McrBC is a two-component MDRS that in Escherichia coli (Ec) restricts phage DNA and foreign DNA containing methylated cytosines. EcMcrB consists of an N-terminal DNA-binding domain that targets fully or hemi-methylated RMC sites (where R is a purine base and MC is a 4-methyl-, 5-methyl-, or 5-hydroxymethyl-cytosine), and a C-terminal AAA+ (extended ATPases Associated with various cellular Activities) domain that hydrolyzes GTP and oligomerizes into hexamers. Biochemical data suggest that stimulated GTP hydrolysis powers DNA translocation, allowing EcMcrBC complexes bound to distant RMC sites to interact and induce cleavage on both strands. Here, we present cryo-EM structures of an McrB hexamer and McrBC complexes from the evolutionarily distant archaeal species Thermococcus gammatolerans (Tg) and the well-characterized E. coli system.

To overcome this limitation, we produced complexes containing full-length TgMcrC bound to the AAA+ domain of TgMcrB (TgMcrBAAAC) in the presence of GTPγS. This assembly was structurally more homogeneous and allowed us to calculate maps of the “half”-complex at 3.7-Å resolution, as well as a C2-symmetrized map of the entire TgMcrBAAAC tetradecameric complex at 4.2-Å resolution. A TgMcrC dimer bridges two TgMcrBAAA hexamers in this structure, with the scaffold and nuclease domains forming the dimer interface. The nuclease domains associate through their α12 helices and a loop between the β10 and β11 strands (“L”), whereas the neighboring scaffold domains interact with each other through their β4 strands that form main-chain hydrogen bonds with each other. Structural superposition confirms TgMcrC’s C terminus shares the same fold and identifies Asp340TgMcrC, Asp354TgMcrC, and Lys356TgMcrC as putative catalytic side chains based on their spatial alignment with the EndoMS metal-binding residues. The nuclease domains align in an orientation that resembles the dimer configuration captured in our cryo-EM structures; however, we observe numerous steric clashes in both models. TgMcrC’s scaffold domain and the α12 nuclease helices collide with the DNA substrate. We therefore speculate that our dimeric McrBC structures depict a conformation that is incompatible with DNA cleavage, and that a major conformational change would be required for nuclease activity to proceed unencumbered. Modeling these interactions in the context of the tetradecameric complexes indicates further steric hindrance: superimposed DNA strands would clash with the McrB subunits and have a trajectory that is directed away from the central pore in the hexamer, offset by nearly 30° and 10° for the TgMcrBAAAC and EcmMCrB∆NC structures, respectively. In support of this notion, we find GDP at the A/B site in our EcMcrBC structure, the F/A site in the structure of the TgMcrBC complex, and at both sites in the structure of the TgMcrBAAAC complex.

>[12x]MNESAGHNIKEDYFRVDMLLNKKGQVILYGPPGTGKTWIARKYVVEETNEKTPGNKWEFITFHQSYSYEEFIEGFRPRTDNEEKIRYVVEDGIFKKIALRALVKGLFELEDATIGKDKIHRLYILLTKKEPLSPTEYEEYLRLKRYLWELVGGLPKDKLKNLTPKFYLIIDEINRGNISKIFGELITLLEKDKRLGGENQLIVRLPYSGEPFAVPPNLYIIGTMNTADRSIALLDVALRRRFAFIEVEPRPEFLEKENLKKIREKKLKTEDRKRLNEKLNELFSKLGNDNYFLKTLLEKINVRITVVKDRDHRIGHSYFLNVETVEDLHHVWYYEVLPLLMEYFYNDWETIKWVLNEKGKEHGNVFFEKLRLTGPNGEEAYQLKVLEGDAFIGALKRIISKNTPSQEGGATTNEENSPENTQSQTEGD;>MPRLTTITLYEHDEKRYRDIAGDKKAIQDALIKLNKQFKKDFKKLDRSEDNSDTEDTIDESKGVVEVYANKIKARHYVGFAAVDNVFLQILPKVFKPKKEQTQETQEDTWEPILAFIRMLDMAYGLKIKDHDLAYLQGRNLRPNLYEVFIYLFAKSLWSEVQRGYHREYVEVHREEKFLRGKLLMSRQIRKLPHQLNTFSVEVHELIEDNLLNRIFYASVREALRRTTWGLNRKLLGELMLAFDGITPIHLRTEHFERVHFTRLNERFRRPFELAKLLFMPASGKGRSREVSGFFVDMNKLFERFIERVLVRNLPPEYKLFYQESYPFLKNQNGSSQKPDYVVRKGNTPVVVLDAKYRELKERIPSSDMLRQLYVYSRIWGYKTSHENDSKPPAVIVIPSSSTYNQGLPDKPLEFEFFDERKLFIVAYNMDYVKTGAIFKADKNFRRSLNNIIGKLNT[2x]> GSMGATKILMDSTHFNEIRSIIRSRSVAWDALARSEELSEIDASTAKALESILVKKNIGDGLSSSNNAHSGFKVNGKTLIPLIHLLSTSDNEDCKKSVQNLIAELLSSDKYGDDTVKFFQEDPKQLEQLFDVSLKGDFQTVLISGFNVVSLLVQNGLHNVKLVEKLLKNNNLINILQNIEQMDTCYVCIRLLQELAVIPEYRDVIWLHEKKFMPTLFKILQRATDSQLATRIVATNSNHLGIQLQYHSLLLIWLLTFNPVFANELVQKYLSDFLDLLKLVKITIKEKVSRLCISIILQCCSTRVKQHKKVIKQLLLLGNALPTVQSLSERKYSDEELRQDISNLKEILENEYQELTSFDEYVAELDSKLLCWSPPHVDNGFWSDNIDEFKKDNYKIFRQLIE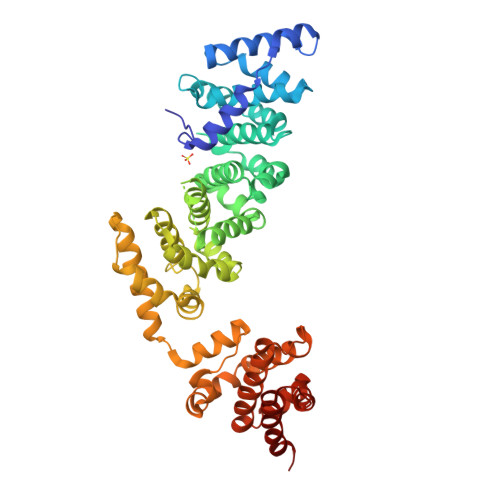LLQAKVRNGDVNAKQEKIIIQVALNDITHVVELLPESIDVLDKTGGKADIMELLNHSDSRVKYEALKATQAIIGYTFK(2~{R})-2-[[(3~{R},4~{R},5~{S})-3,4,5,6-tetrakis(oxidanyl)-2-oxidanylidene-hexyl]amino]pentanedioic 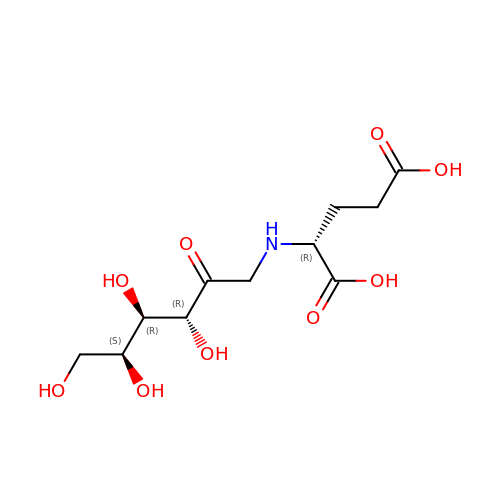acid | C11 H19 N O9 | PUFNBARRTADWAC-XWPZMVOTSA-N>[3x]MSQSSRLSALPIFQASLSASQSPRYIFSSQNGTRIVFIQDNIIRWYNVLTDSLYHSLNFSRHLVLDDTFHVISSTSGDLLCLFNDNEIFVMEVPWGYSNVEDVSIQDAFQIFHYSIDEEEVGPKSS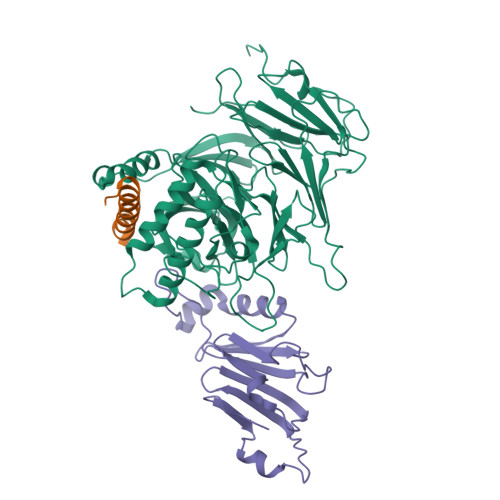IKKVLFHPKSYRDSCIVVLKEDDTITMFDILNSQEKPIVLNKPNNSFGLDARVNDITDLEFSKDGLTLYCLNTTEGGDIFAFYPFLPSVLLLNEKDLNLILNKSLVMYESLDSTTDVIVKRNVIKQLQFVSKLHENWNSRFGKVDIQKEYRLAKVQGPFTINPFPGELYDYTATNIATILIDNGQNEIVCVSFDDGSLILLFKDLEMSMSWDVDNYVYNNSLVLIERVKLQREIKSLITLPEQLGKLYVISDNIIQQVNFMSWASTLSKSINESDLNPLAGLKFESKLEDIATIERIPNLAYINWNDQSNLALMSNKTLTFQNISS;>[3x]GPHSSITKDMKGFKVVEVGLAMNTKKQIGDFFKNLNMAK;>[3x]GPHAGIVLTKVGYYTIPSMDDLAKITNEKGECIVSDFTIGRKGYGSIYFEGDVNLTNLNLDDIVHIRRKEVIVYVDDNQKPPVGEGLNRKAEVTLDGVWPTDKTSRCLIKSPDRLADINYEGRLEAVSRKQGAQFKEYRPETGSWVFKVSHF>GSNNELYLELMKLREHSDQHVKELKTSLKKCARETADLKFLNNQYAHKLKLLEKESKAKNERIQ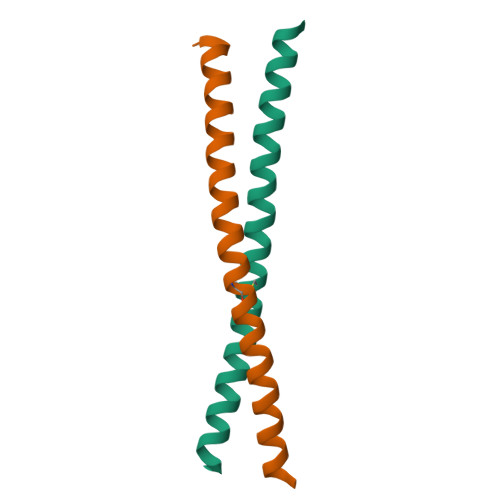Q[2x]> GSHMAASATAAAVAAEVISVHSLEQWTMQIEEANTAKKLVVIDFTASWCGPSRIMAPVFADLAKKFPNAVFLK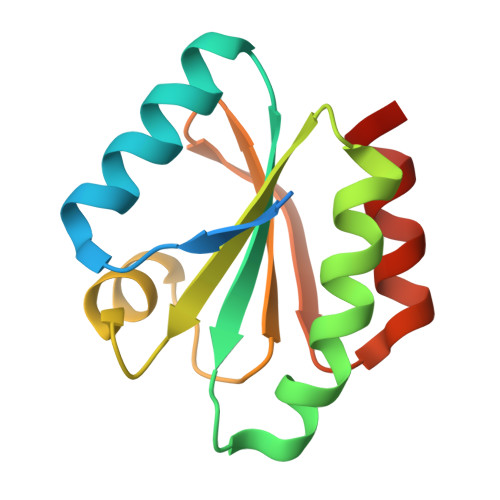VDVDELKPIAEQFSVEAMPTFLFMKEGDVKDRVVGAIKEELTAKVGLHAAAQ> CPAR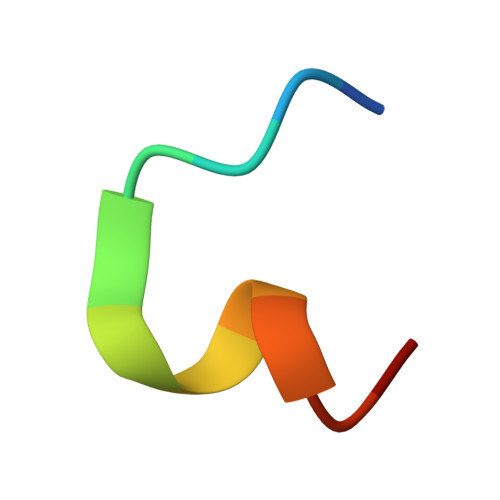YGWDYECX UDG is exquisitely selective for uracil bases located in single- or double-stranded DNA, and it selectively removes uracil by cleaving the N-glycosyl linkage between the base and the deoxyribose, leaving behind an abasic site. As previously reported, UDG forms a single domain structure consisting of an initial left-handed coil of helices followed by a β−α−β structure that forms an internal four-stranded parallel β-sheet with external α-helices. The p56 monomer comprises a three-stranded antiparallel β-sheet with a helix lying along it. The biological dimer is observed to form a six-membered sheet with the helices lying against one another forming a single hydrophobic core.

Protein p56 of bacteriophage PZA, when co-expressed with HHV-1 UDG in E. coli, appeared to form a stable complex. Reminiscent of inhibition by ugi, the UDG active site is occupied by p56. However, where ugi achieves this blockade with a distorted edge-on beta strand, p56 almost exclusively uses the alpha helix of one of its monomeric subunits (molecule C). Contacts to the UDG DNA-binding cleft from this p56 helix span Ser32 through Asn42. Several hydroxyl and backbone oxygen interactions closely resemble those formed by the phosphates of the DNA backbone in the kinked conformation exhibited when the uracil base is flipped out. The tightest point of interaction in the p56 complex appears to be the minor groove intercalation loop of UDG. The apical leucine residue fits into a deep pit between the two helices of the inhibitor dimer. This box-sided pit is formed by a rigid interaction of mutually perpendicular pairs of residues from each p56 subunit helix. Glu37 and Tyr40 side chains from p56 molecules C and D, form the walls of the box. In the apo form of HHV-1 UDG, Leu214 adopts a conformation similar to that observed in the described complex with p56, with a shift of 0.5 Å in Cα position but with a similar sidechain conformation; this conformation is also similar in apo human UDG.

>STGGVSPAATSAPLDWTTFRRVFLIDDAWRPLMEPELANPLTAHLLAEYNRRCQTEEVLPPREDVFSWTRYCTPDEVRVVIIGQDPYHHPGQAHGLAFSVRANVPPPPSLRNVLAAVKNCYPEARMSGHGCLEKWARDGVLLLNTTLTVKRGAAASHSRIGWDRFVGGVIRRLAARRPGLVFMLWGTHAQNAIRPDPRVHCVLKFSHPSPLSKVPFGTCQHFLVANRYLETRSISPIDWSV[2x];>[4x]VQNDFLDSYDVTMLLQDDNGKQYYEYHKGLSLSDFEVLYGNTVDEIIKLRVDKIS(1,4-diazepane-1,4-diyl)di(propane-3,1-diyl) bis(3,4,5-trimethoxybenzoate) | C31 H44 N2 O10 | 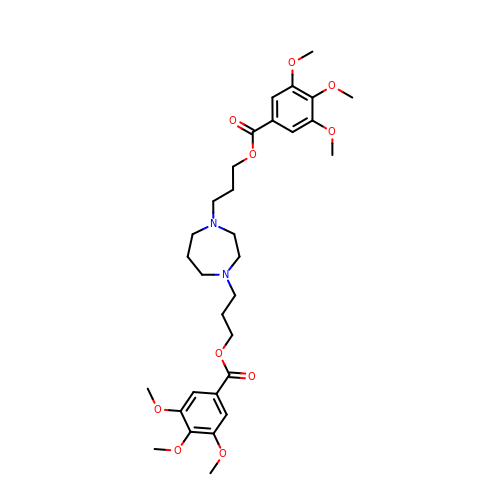QVZCXCJXTMIDME-UHFFFAOYSA-N>[6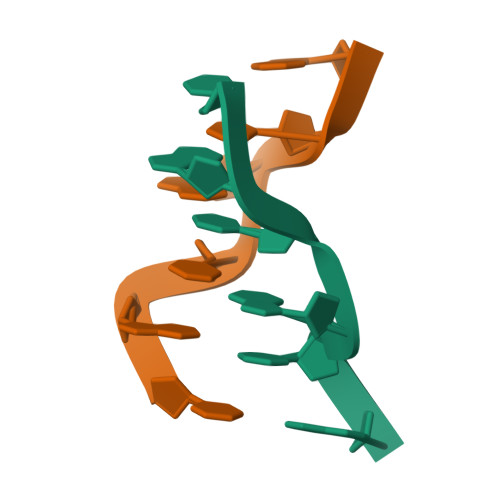x]CGCGCG>[2x]GSHMNGLIYAVGGYDGNTHLNSVEAYDPERNEWSLVAPLSTRRSGVGVAVLNGLIYAVGGYDGNTHLNSVEAYDPHHNEWSLVAPLSTRRSGVGVAVLNGLIYAVGGYDGNTHLNSVEAYDPERNEWSLVAPLSTRRSGVGVAVLNGLIYAVGGYDGNTHLNSVEAYDPHHNEWSLVAPLSTRRSGVGVAVLNGLIYAVGGYDGNTHLNSVEAYDPERNEW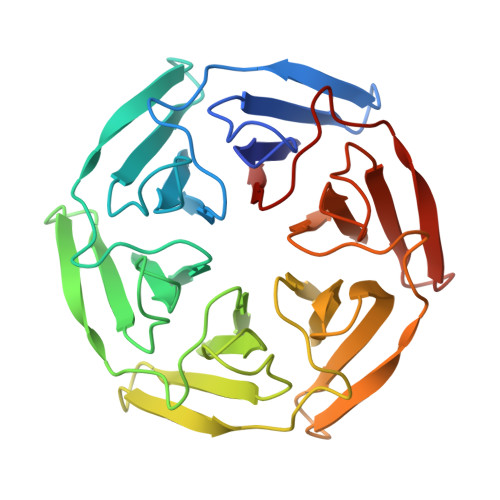SLVAPLSTRRSGVGVAVLNGLIYAVGGYDGNTHLNSVEAYDPHHNEWSLVAPLSTRRSGVGVAVL>[2x]LILDFNKVQMRSQQLAPGVYAHLPADSAELNAKGGVAGTSG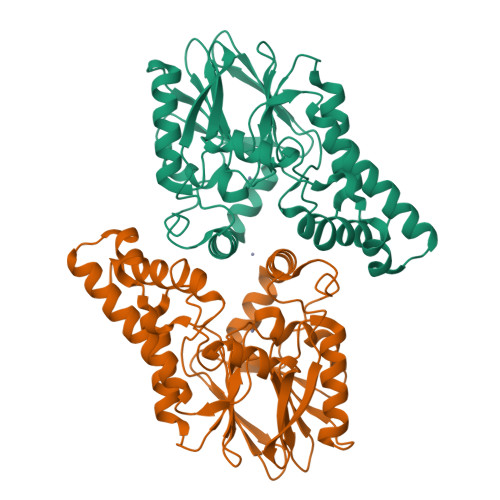GLIVGTRGAMLIETMLNRRLFDQVQALAKKEALGLPLLYAVNTSYHGDHSYGNMYLKAPTRVIQSTKTRDYVDGHLADDKAFMVKNFGAGRGVEQITARTGDILVPPGGRVSVDLGGKTVEIIDFGFAQTGGDLFVWEPQSKVMWTGNAVVASKPALPWLLDGKLVETLATLQKVYDFLPPDATIVPGHGVPMAREGLRWHLDYLAAVQAGVKDALARKLSLEQTVTELKMPEFRGYVLFDFVHPDLNVPAAYENLYFQ1-(5-bromanylpyridin-2-yl)-3-(2-hydroxyethyl)urea | C8 H10 Br N3 O2 | 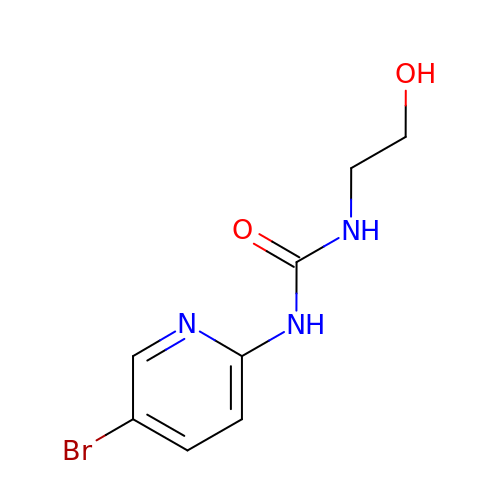DWHYNYBZZGQFNY-UHFFFAOYSA-N> MKLFRVVKRGYYISYAILDNSTIIRLDEDPIKALMRYSENKEVLGDRVTGIDYQSLLKSFQINDIRITKPIDPPEVWGSGISYEMARERYSEENVAKILGKTIYEKVYDAVRPEIFFKATPNRCVGHGEAIAVRSDSEWTLPEPELAVVLDSNGKILGYTIMDDVSARDLEAENPLYLPQSKIYAGCCAFGPVIVTSDEIKNPYSLDITLKIVREGRVFFEGSVNTNKMRRKIEEQIQYLIRDNPIPDGTILTTGTAIVPGRDKGLKDEDIVEITISNIGTLITPVKKR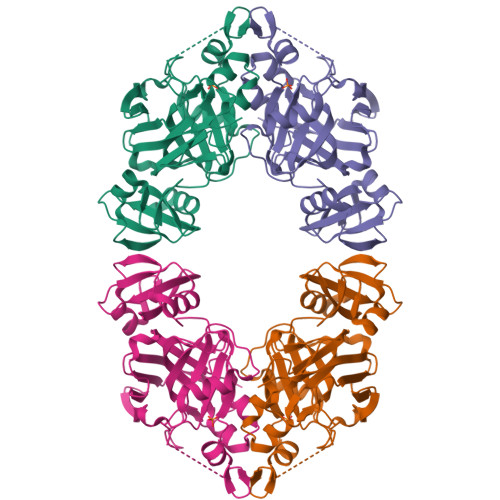RKIT>[2x]PKGTFKDYV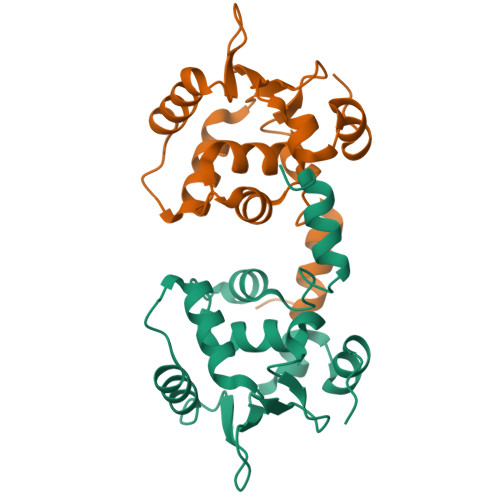RDRADLNKDKPVIPAAALAGYTGSGPIQLWQFLLELLTDKSCQSFISWTGDGWEFKLSDPDEVARRWGKRKNKPKMNYEKLSRGLRYYYDKNIIHKTAGKRYVYRFVCDLQSLLGYTPEELHAMLDVKPDAD>[2x]MDYKDDDDKAVFSKLQLLGQAIPPKQYAPGVVGMLAVFALIKLYKQDIRGTKHLVAKTKEGKKERAVVDKVFFSRLIQILKIMVPRTFCKETGYLVLIAVMLVSRTYCDVWMIQNGTLIESGIIGRSRKDFKRYLLNFIAAMPLISLVNNFLKYGLNELKLCFRVRLTKYLYEEYLQAFTYYKMGNLDNRIANPDQLLTQDVEKFCNSVVDLYSNLSKPFLDIVLYIFKLTSAIGAQGPASMMAYLVVSGLFLTR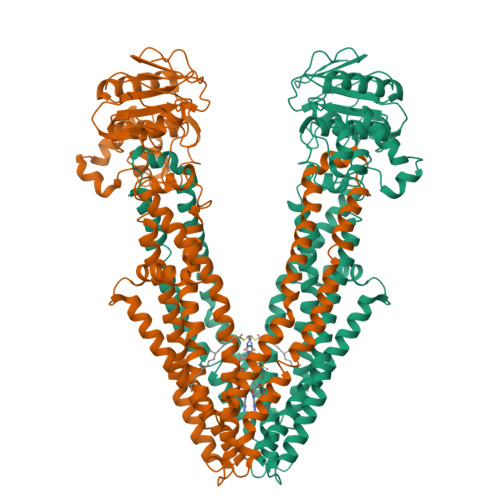LRRPIGKMTITEQKYEGEYRYVNSRLITNSEEIAFYNGNKREKQTVHSVFRKLVEHLHNFILFRFSMGFIDSIIAKYLATVVGYLVVSRPFLDLSHPRHLKSTHSELLEDYYQSGRMLLRMSQALGRIVLAGREMTRLAGFTARITELMQVLKDLNHGKYERTMVSQQEKGIEGVQVIPLIPGAGEIIIADNIIKFDHVPLATPNGDVLIRDLNFEVRSGANVLICGPNGCGKSSLFRVLGELWPLFGGRLTKPERGKLFYVPQRPYMTLGTLRDQVIYPDGREDQKRKGISDLVLKEYLDNVQLGHILEREGGWDSVQDWMDVLSGGEKQRMAMARLFYHKPQFAILDECTSAVSVDVEGYIYSHCRKVGITLFTVSHRKSLWKHHEYYLHMDGRGNYEFKQITEDTVEFGS Ketoacyl-acyl carrier protein reductases (FabG; EC 1.1.1.100) are highly conserved and ubiquitously expressed enzymes of the bacterial type II fatty acid synthesis (FASII) pathway, catalysing the reduction of the acyl carrier protein (ACP) linked β-ketoacyl molecules to β-hydroxyacyl-ACP thioesters necessary for the formation of saturated and unsaturated fatty acids. FabG enzymes are members of the short-chain alcohol dehydrogenase/reductase (SDR) family (also known as the short chain oxidoreductase or SCOR family). The refined structures of the two crystal forms of YpFabG reveal that the protein contains a typical Rossmann fold motif, comprised of a seven strand twisted β-sheet surrounded by eight α-helices. The YpFabG tetramer is formed through two types of interfaces.

Recombinant YpFabG crystallised in two different crystal forms; YpFabG crystallised in the presence of TMAO (YpFabG TMAO) diffracted to 2.5 Å and contained one monomer in the ASU, with electron density visible for 234 of 244 residues (residues 2–189, and 197–241), and was refined to Rwork/Rfree values of 0.220/0.255. Despite very similar crystallisation conditions, the YpFabG TMAO crystal displays P42212 symmetry with a single YpFabG monomer within the ASU, whereas the YpFabG NaBr crystal displays P1211 symmetry with four YpFabG monomers within the ASU arranged to form a homotetramer. Overall, these secondary structure elements are arranged in a topology of β1-α1-β2-α2-β3—α3—β4-α4-β5-α5-β6—α6-α7-α8-β8. These secondary structure elements are clearly observable in the YpFabG TMAO structure, with only residues 190–197, which form part of the helix-turn-helix motif comprised of helices α6 and α7, and the loop region connecting the two helices, unmodelled due to disorder. Furthermore, the loop joining β-strand β5 and α-helix α5 within the YpFabG NaBr structure is largely disordered, with superposition of NADP+ bound and unbound E. coli FabG structures indicating that Ser138 located at the start of this loop region must move ~3 Å to accommodate the nicotinamide portion of NADP+. In comparison, this region is ordered within the YpFabG TMAO structure, and adopts a conformation almost identical to that of E. coli FabG in complex with NADP+. The conformation that appears to mimic that of E. coli FabG in complex with NADP+ could possibly be induced by crystal contacts, or the presence of TMAO within a binding pocket that becomes occupied by the 2’-phosphate of NADPH upon co-factor binding. Crystallographic symmetry of YpFabG TMAO arrange to form a tetramer highly similar to that within the ASU of YpFabG NaBr, with superposition of the YpFabG NaBr structure and the tetramer of YpFabG TMAO generated through crystallographic symmetry indicating no clashes that would alter crystal packing.

> MSFEGKIALVTGASRGIGRAIAELLVERGACVIGTATSEKGAEAISAYLGENGKGLMLNVVDPTSIDTVLATIRAEFGEVDILVNNAGITRDNLLMRMKDDEWQDIIDTNLTSVFRLSKAVMRAMMKKRFGRIITIGSVVGTMGNAGQVNYAAAKAGVIGFSKSLAREVASRGITVNVVAPGFIETDMTRTLTDDQRAGILAQVPANRLGDAKEIASAVAFLASDEASYISGETLHVNGGMYMI> GSHMKRNYILGLDIGITSVGYGIIDYETRDVIDAGVRLFKEANVENNEGRRSKRGARRLKRRRRHRIQRVKKLLFDYNLLTDHSELSGINPYEARVKGLSQKLSEEEFSAALLHLAKRRGVHNVNEVEEDTGNELSTKEQISRNSKALEEKYVAELQLERLKKDGEVRGSINRFKTSDYVKEAKQLLKVQKAYHQLDQSFIDTYIDLLETRRTYYEGPGEGSPFGWKDIKEWYEMLMGHCTYFPEELRSVKYAYNADLYNALNDLNNLVITRDENEKLEYYEKFQIIENVFKQKKKPTLKQIAKEILVNEEDIKGYRVTSTGKPEFTNLKVYHDIKDITARKEIIENAELLDQIAKILTIYQSSEDIQEELTNLNSELTQEEIEQISNLKGYTGTHNLSLKAINLILDELWHTNDNQIAIFNRLKLVPKKVDLSQQKEIPTTLVDDFILSPVVKRSFIQSIKVINAIIKKYGLPNDIIIELAREKNSKDAQKMINEMQKRNRQTNERIEEIIRTTGKENAKYLIEKIKLHDMQEGKCLYSLEAIPLEDLLNNPFNYEVDHIIPRSVSFDNSFNNKVLVKQEEASKKGNRTPFQYLSS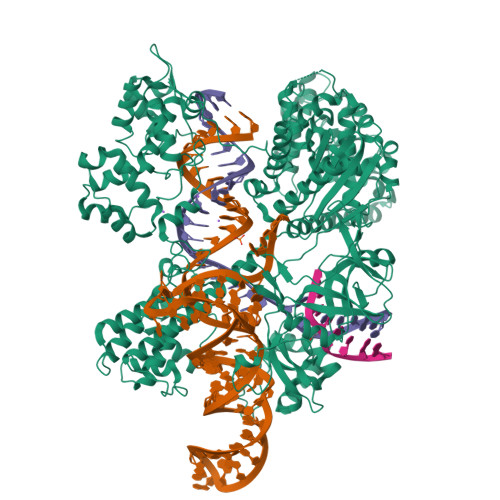SDSKISYETFKKHILNLAKGKGRISKTKKEYLLEERDINRFSVQKDFINRNLVDTRYATRGLMNLLRSYFRVNNLDVKVKSINGGFTSFLRRKWKFKKERNKGYKHHAEDALIIANADFIFKEWKKLDKAKKVMENQMFEEKQAESMPEIETEQEYKEIFITPHQIKHIKDFKDYKYSHRVDKKPNRELINDTLYSTRKDDKGNTLIVNNLNGLYDKDNDKLKKLINKSPEKLLMYHHDPQTYQKLKLIMEQYGDEKNPLYKYYEETGNYLTKYSKKDNGPVIKKIKYYGNKLNAHLDITDDYPNSRNKVVKLSLKPYRFDVYLDNGVYKFVTVKNLDVIKKENYYEVNSKAYEEAKKLKKISNQAEFIASFYNNDLIKINGELYRVIGVNNDLLNRIEVNMIDITYREYLENMNDKRPPRIIKTIASKTQSIKKYSTDILGNLYEVKSKKHPQIIKKG>MAKKTSSKPTDPPVYPVTVPFLGHIVQFGKNPLEFMQRCKRDLKSGVFTISIGGQRVTIVGDPHEHSRFFSPRNEILSPREVYTIMTPVFGEGVAYAAPYPRMREQLNFLAEELTIAKFQNFVPAIQHEVRKFMAENWKEDEGVINLLEDCGAMIINTACQCLFGEDLRKRLNARHFAQLLSKMESSLIPAAVFMPWLLRLPLPQSARCREARAELQKILGEIIVAREKEEASKDNNTSDLLGGLLKAVYRDGTRMSLHEVCGMIVAAMFAGQHTSTITTSWSMLH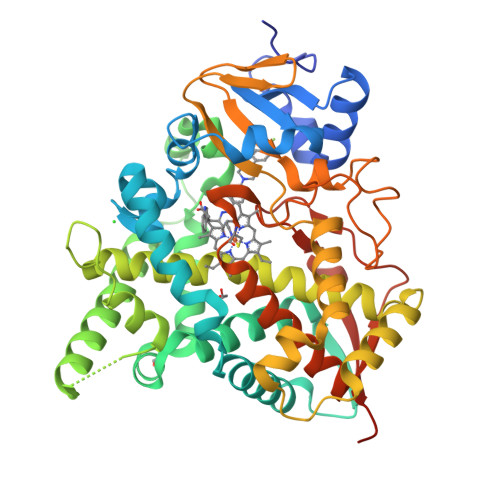LMHPKNKKWLDKLHKEIDEFPAQLNYDNVMDEMPFAERCVRESIRRDPPLLMVMRMVKAEVKVGSYVVPKGDIIACSPLLSHHDEEAFPNPRLWDPERDEKVDGAFIGFGAGVHKCIGQKFALLQVKTILATAFREYDFQLLRDEVPDPDYHTMVVGPTLNQCLVKYTRKKKLPSHHHHHH[2x]>GSNFCDSKCKLRCSKAGLADRCLKFCGICCEECKCVPSGTYGNKHECPCYRDKKNSKGKSKCP[2x];>[2x]GSNFCDSKCKLRCSKAGLADRCLKYCGIC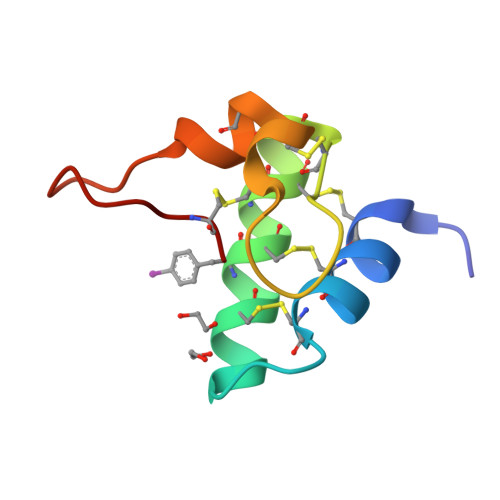CEECKCVPSGTYGNKHECPCYRDKKNSKGKSKCP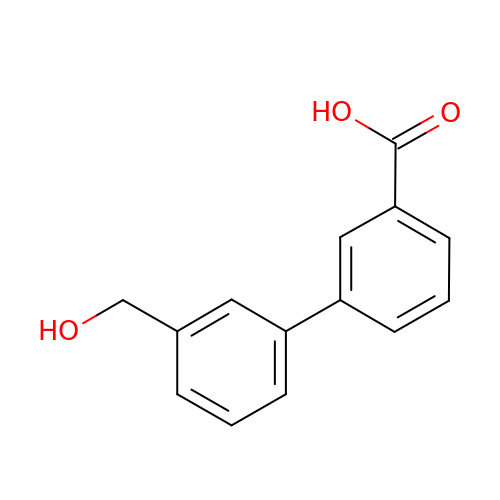3-[3-(hydroxymethyl)phenyl]benzoic acid | C14 H12 O3 | SWVDMIKPVOEKNC-UHFFFAOYSA-N> GPMDFLRSLDWTQVIAGQYVSNPRFNISDYFEIVRQPGDGNCFYHSIAELTMPNKTDHSYHYIKRLTESAARKYYQEEPEARLVGLSLEDYLKRMLSDNE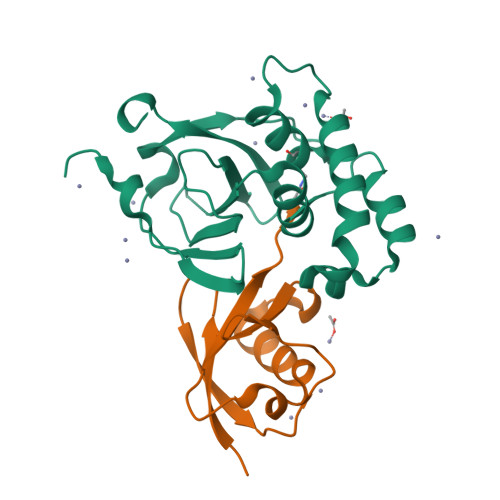WGSTLEASMLAKEMGITIIIWTVAASDEVEAGIKFGDGDVFTAVNLLHSGQTHFDALRILPQFETDTREALSLMDRVIAVDQLTS;> MDEPLSILVRNNKGRSSTYEVRLTQTVAHLKQQVSGLEGVQDDLFWLTFEGKPLEDQLPLGEYGLKPLSTVFMNLRLRG> APDTSVSNKQNFSTDVIYQIFTDRFSDGNPANNPTGAAFDGTCTNLRLYCGGDWQGIINKINDGYLTGMGVTAIWISQPVENIYSIINYSGVNNTAYHGYWARDFKKTNPAYGTIADFQNLIAAAHAKNIKVIIDFAPNHTSPASSDQPSFAENGRLYDNGTLLGGYTNDTQNLFHHNLGTDFSTTENGIYKNLYDLADLNHNNSTVDVYLKDAIKMWLDLGIDGIRMDAVKHMPFGWQKSFMAAVNNYKPVFTFGEWFLGVNEVSPENHKFANESGMSLLDFRFAQKVRQVFRDNTDNMYGLKAMLEGSAADYAQVDDQVTFIDNH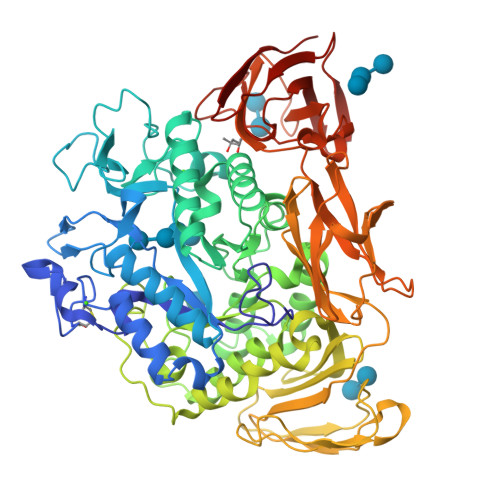DMERFHASNANRRKLEQALAFTLTSRGVPAIYYGTEQYMSGGTDPDNRARIPSFSTSTTAYQVIQKLAPLRKCNPAIAYGSTQERWINNDVLIYERKFGSNVAVVAVNRNLNAPASISGLVTSLPQGSYNDVLGGLLNGNTLSVGSGGAASNFTLAAGGTAVWQYTAATATPTIGHVGPMMAKPGVTITIDGRGFGSSKGTVYFGTTAVSGADITSWEDTQIKVKIPAVAGGNYNIKVANAAGTASNVYDNFEVLSGDQVSVRFVVNNATTALGQNVYLTGSVSELGNWDPAKAIGPMYNQVVYQYPNWYYDVSVPAGKTIEFKFLKKQGSTVTWEGGSNHTFTAPSSGTATINVNWQP> SGWHRRT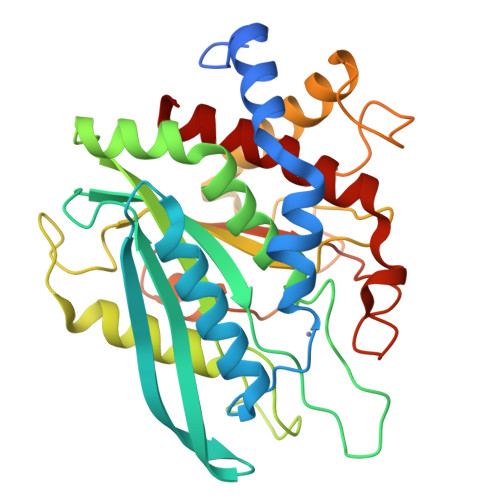EELPLGRELRVPLIGSLPEARLRRVVGQLDPQRLWSTYLRPLLVVRTPGSPGNLQVRKFLEATLRSLTAGWHVELDPFTASTPLGPVDFGNVVATLDPRAARHLTLACHYDSKLFPPGSTPFVGATDSAVPCALLLELAQALDLELSRAKKQAAPVTLQLLFLDGEEALKEWGPKDSLYGSRHLAQLMESIPHSPGPTRIQAIELFMLLDLLGAPNPTFYSHFPRTVRWFHRLRSIEKRLHRLNLLQSHPQEVMYFQPGEPFGSVEDDHIPFLRRGVPVLHLISTPFPAVWHTPADTEVNLHPPTVHNLCRILAVFLAEYLGL>[2x]MGLAVFLPPYPFRGLKAPYLWMFYKYLHCATDSILFITGEDYLSVTDDEAQRARWEFDPASMASLGYELPNAQSMACHEYLTLDNAFYETLLSRHHHDPIKSFSAFLTERIPDLETELHALLDSKKGIIDQIDTFISICNCPSLEHVARTLGKEVMHIEIGPLRAPMYRNTAYLDFAGVNGGTEASARYEKCQAEFDIKASLGDLHNYFLEVLPPAEAATHSAAGVVLQVEDNSNLIAYNHDFTNISLLSYVRQRYEKEDILVRAHPGSLFRLRDDVFTIDDSANSLAFINQCNEVFTINSSVGLEAILTGKKTTVLGDCSYAFINELAGASATVNAAAFYLFSYLVPFDLVFNQEYLKFRLGHPEEREIVGKHIEFYSADMPGSLSQAAHSLSSLINEAISLEHHHHHH

WbbB, a lipopolysaccharide O-antigen synthesis enzyme from Raoultella terrigena, contains an N-terminal glycosyltransferase domain with a highly modified architecture that adds a terminal β-Kdo (3-deoxy-d-manno-oct-2-ulosonic acid) residue to the O-antigen saccharide, with retention of stereochemistry. WbbB’s two C-terminal GT domains produce a polymer with a [4)-α-Rhap-(1→3)-β-GlcpNAc-(1→] repeat unit, while the N-terminal domain of the protein contains a GT99 retaining β-Kdo transferase, referred to here as WbbBGT99. Kdo addition blocks further polymerization while creating the epitope recognized by the carbohydrate-binding module of the cognate ABC transporter, allowing export prior to ligation to lipid A-core in the periplasm. The evidence presented above strongly argues that WbbBGT99 is a retaining glycosyltransferase that uses a double-displacement mechanism analogous to that used by retaining glycoside hydrolases.

Capturing WbbBGT99 in complex with the CMP-β-Kdo donor is complicated by its instability. The density corresponding to the Kdo group is significantly weaker than that for the nucleotide but refinement of the structure using both CMP and CMP-β-Kdo results in 25% occupancy of CMP-β-Kdo in the active site, with atomic displacement parameters (ADPs; B-factors) similar to surrounding residues. In WbbBGT99, the CMP-β-Kdo density is not consistent with this conformation, with Kdo instead refining to the higher-energy skew-boat (OS3) conformation. The C1 carboxylate group forms hydrogen bonds with both the backbone and side chain amide of the invariant Gln228 from the QxxxD motif. In addition, O4 forms hydrogen bonds with Arg163, as well as the phosphate-linking oxygen, while O5 and O7 form a hydrogen bond but are otherwise facing the solvent channel. The exocyclic O8 hydroxyl group hydrogen bonds to both Glu158 and Asn179. In this conformation, Asn232(=Asp) packs against the edge of the carboxylate and the exposed ring of Kdo, but interacts only with aliphatic groups and makes no hydrogen bonds. Notably, both polar atoms are within van der Waals contact distance of the anomeric carbon (the closer is 3.8 Å away) and can be brought closer (to within 2.8 Å) by rotation around the Cβ–Cγ bond. The anomeric carbon is therefore completely buried in this conformation, precluding (absent a major reorganization of the active site) the acceptor approaching this atom as required for an SNi reaction.> MVVKVYGPAVAVCPQRVMACLLEKGVEFDLVHVDLDSGEQKLPEFLLKQPFGQVPVVEDGDFKLFESRAIIRYYAAKYEDRGPNLLGNTLEEKALVDQWLEIEAHNFNDLVFNIVFQVVILPRIGQQGDSELVRTYEEKLEKVLDVYEKRLSKSKYLAGDSFTLADLSHLPATRYLVNEAGLGHLVKDRKKLNAWWEDISSRPAWKKLMNLAGF

Through biochemical and structural analysis, here we show that anthocyanin-related glutathione transferases, currently implicated only in anthocyanin transport, catalyse an essential dehydration of the leucoanthocyanidin dioxygenase product, flavan-3,3,4-triol, to generate cyanidin. Using PtGSTF8 from poplar as a model enzyme, we use biochemical, structural and computational methods to demonstrate that arGSTs employ a GSH-dependent Brønsted base mechanism for conversion of the LDOX product flavan-3,3,4-triol or flavan-3-on-4-ol into flav-2-en-3,4-diol (8-B4), an equilibrium form of cyanidin. Based on the here-presented biochemical, structural and computational evidence, we propose that arGSTs utilize a GSH-dependent Brønsted base mechanism for conversion of the semi-stable LDOX product flavan-3,3,4-triol or flavan-3-on-4-ol into flav-2-en-3,4-diol (8-B4), the 4-hydration species of cyanidin.

To better understand the catalytic machinery of arGSTs, we determined the crystal structure of PtGSTF8 as a ternary complex with GSH and the substrate analogue (−)-catechin to a resolution of 1.09 Å. The structure comprises the typical GST fold with an N-terminal thioredoxin-like domain (β1α1β2α2β3β4α3) and an all-helical C-terminal domain (α4α5α6α7α8). The active-site cavity, which is located between the two domains, comprises a glutathione binding site (G-site), formed mainly by the N-terminal domain, and a hydrophobic substrate-binding site (H-site), which is formed by the C-terminal domain. However, presumably to accommodate (−)-catechin, the active site is substantially enlarged by a shift of the α4′′ and α4′′′ helices by up to 1.71 Å and an upwards movement of the side chain of phenylalanine F112. Within the H-site, the substrate analogue interacts through hydrogen bonds to N108 and the backbone of V12, a π–π interaction with F112, water bridges to R16 and Y175, and hydrophobic interactions with V12 and V115. Interestingly, the amino acid composition of the substrate-binding H-site and the G-site, which binds to GSH through hydrogen bonds and salt bridges, is strikingly uniform amongst arGSTFs, making the existence of similar substrate–enzyme interactions in other arGSTFs plausible. To shed light on the interactions of the enzyme with the natural substrates, we docked flavan-3,3,4-triol and flavan-3-on-4-ol into the active pocket of the crystal structure of PtGSTF8 obtained with (−)-catechin. The best binding poses for both substrates had a highly similar conformation to (−)-catechin, with an RMSD of matched atoms of 0.51 Å for flavan-3,3,4-triol and 0.54 Å for flavan-3-on-4-ol. The docking analyses revealed that the positioning of the GSH-thiolate in relation to C-2 and O-3 of the docked substrates could enable an acid–base mechanism of dehydration or tautomerization, in which the GSH cofactor acts as a proton-relay system.> VGSLNCIVAVSQNMGIGKNGDRPWPPLRNEFRYFQRMTTTSSVEGKQNLVIMGKKTWFSIPEKNRPLKGRINLVLSRELKEPPQGAHFLSRSLDDALKLTEQPELANKVDMVWIVGGSSVYKEAMNHP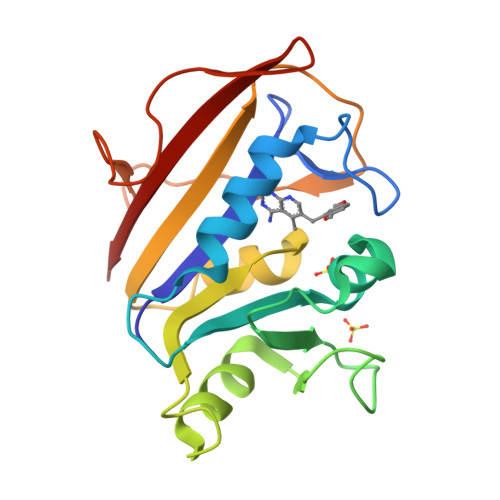GHLKLFVTRIMQDFESDTFFPEIDLEKYKLLPEYPGVLSDVQEEKGIKYKFEVYEKND> ASTSCNVVLTDSQGSFTSPCYPNDYPPSQSCNWTIQAPAGFIVQITFLDFELEEAQGCIYDRVVVKTGTSDAKFCGLTANGLTLNSTGNVMEVFFNSDFSVQKKGFHISYKQVAVTLRNQKVTMPKSSKTILRVSNSISIPVLTAFTVCFEIARTAQKATETIFTLSDAAGTSILAFEKTSNGMELFIGASYCSVDNFLTSSDITATMKPLCLTWTKSSGLIGVYFEGHYFSSICSASQIYTLQSGGLLQIAGKGSSSVSVDDQNLDGFIYNFRLWDHAMLSSELSALTCDTVGNVVDWDHSYWTIPGSSTQTDSTLSCSTAITTLSPGTAGCASGLGCPEDIFYRSTLVVTDEQTPDRDATAIISQWLNQTFQNWMYRVYVDGISLQLITVLSRITTTRQIYLALLVYKNTTDVNLAEVEIESMLRSAPAIGNGLTLDSVTVNLMENCQADEFPVHYRWPESRPTVTQYVPCFPYKDRNASRTCMINRDNYTSFWALPDRGNCTNITSITVSQENAMDVAVQLADISNNGLSKEELTQVVTKVMELVNIAKINATLASTVVTIISNVMVSSEDAQKDASETALKAVDELVQKIEFDGPSLTISSKNLVVGVSALDTTNFNGSTLSAFIATNTTDPQIDFD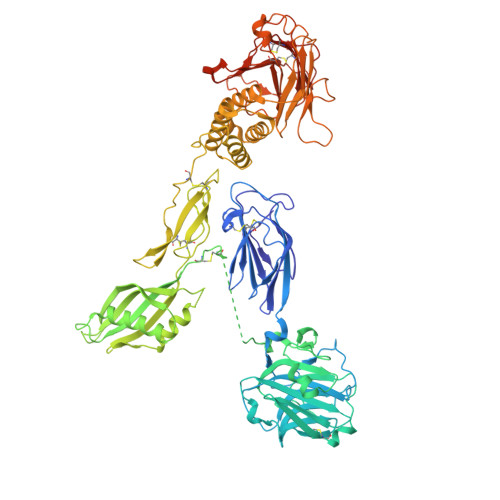SEAHNALAVVTLPPTLLQNLSLSQIEKVSRINFMFFGRTGLFQDHQNNGLTLNSYVVASSVGNFTIKNLQDPVRIEIAHLEYQKDPNPQCVFWDFNLQNYSGGWNSDGCKVGSDSNSNRTVCLCNHLTHFGILMDVSRAHHHHHHHH> RGSSSGDPRADPRIEASRERRALEEAPRREGGPTERKPWGDQYDYLNTRPAELVSKKGTDGVPVMLQTNFFRLKTKPEWRIVHYHVEFEP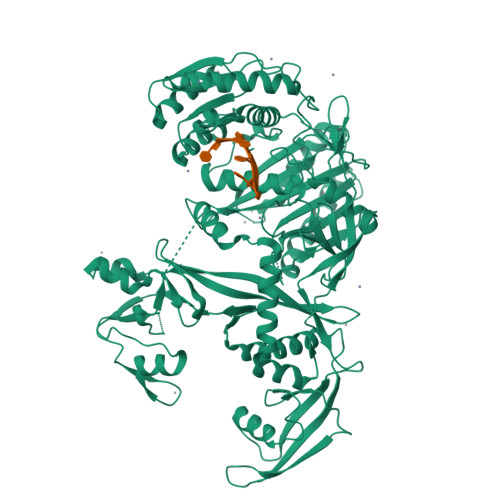SIENPRVRMGVLSNHANLLGSGYLFDGLQLFTTRKFEQEITVLSGKSKLDIEYKISIKFVGFISCAEPRFLQVLNLILRRSMKGLNLELVGRNLFDPRAKIEIREFKMELWPGYETSIRQHEKDILLGTEITHKVMRTETIYDIMRRCSHNPARHQDEVRVNVLDLIVLTDYNNRTYRINDVDFGQTPKSTFSCKGRDISFVEYYLTKYNIRIRDHNQPLLISKNRDKALKTNASELVVLIPELCRVTGLNAEMRSNFQLMRAMSSYTRMNPKQRTDRLRAFNHRLQNTPESVKVLRDWNMELDKNVTEVQGRIIGQQNIVFHNGKVPAGENADWQRHFRDQRMLTTPSDGLDRWAVIAPQRNSHELRTLLDSLYRAASGMGLRIRSPQEFIIYDDRTGTYVRAMDDCVRSDPKLILCLVPNDNAERYSSIKKRGYVDRAVPTQVVTLKTTKNRSLMSIATKIAIQLNCKLGYTPWMIELPLSGLMTIGFDIAKSTRDRKRAYGALIASMDLQQNSTYFSTVTECSAFDVLANTLWPMIAKALRQYQHEHRKLPSRIVFYRDGVSSGSLKQLFEFEVKDIIEKLKTEYARVQLSPPQLAYIVVTRSMNTRFFLNGQNPPPGTIVDDVITLPERYDFYLVSQQVRQGTVSPTSYNVLYSSMGLSPEKMQKLTYKMCHLYYNWSGTTRVPAVCQYAKKLATLVGTNLHSIPQNALEKKFYYL> GMSTAAESEIRQLIERWMQAVRDRDIPGIIAPYADDIVAFDAIQALQFKGKSAYTAHWEMCMGMCTGPMVFELAQLTVHAAGDLALAHWLNRCGPGDDESQCGFMRATVGYR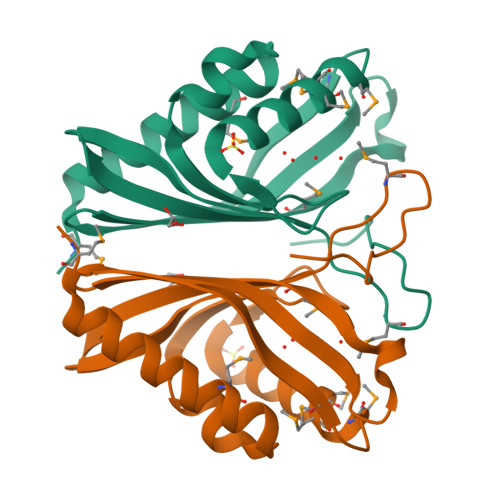RQGGQWQVIHEHWSAPFDMETQKALFDLKP> MTGSLNRHSLLNGVKKMRIILCDTNEVVTNLWQESIPHAYIQNDKYLCIHHGHLQSLMDSMRKGDAIHHGHSYAIVSPGNSYGYLGGGFDKALYNYFGGKPFETWFRNQLGGRYHTVGSATVVDLQRCLEEKTIECRDGIRYIIHVPTVVAPSAPIFNPQNPLKTGFEPVFNAMWNA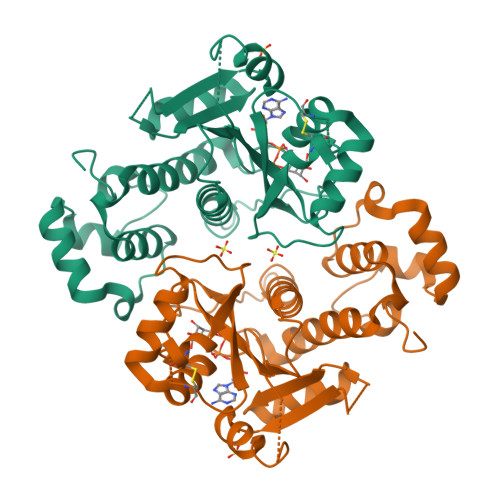LMHSPKDIDGLIIPGLCTGYAGVPPIISCKSMAFALRLYMAGDHISKELKNVLIMYYLQYPFEPFFPESCKIECQKLGIDIEMLKSFNVEKDAIELLIPRRILTLDL> VIEKRIVIDGDGDIDHDQALAQAIRE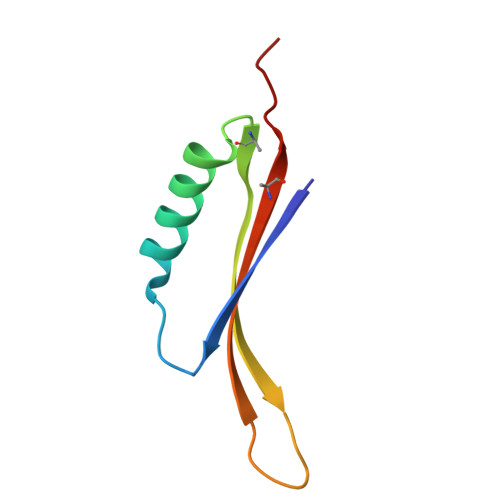AREQHPDMSVTRVVVNKETELAEEGEDRTRQIINITMTKKLDVW>[10x]MSGTEEAILGGRDSHPAAGGGSVLCFGQCQYTAEEYQAIQKALRQRLGPEYISSRMAGGGQKVCYIEGHRVINLANEMFGYNGWAHSITQQNVDFVDLNNGKFYVGVCAFVRVQLKDGSYHEDVGYGVSEGLKSKALSLEKARKEAVTDGLKRALRSFGNALGNCILDKDYLRSLNKLPRQLPLEVDLTKAKRQDLEPSVEEARYNSCRPNMALGHPQLQQVTS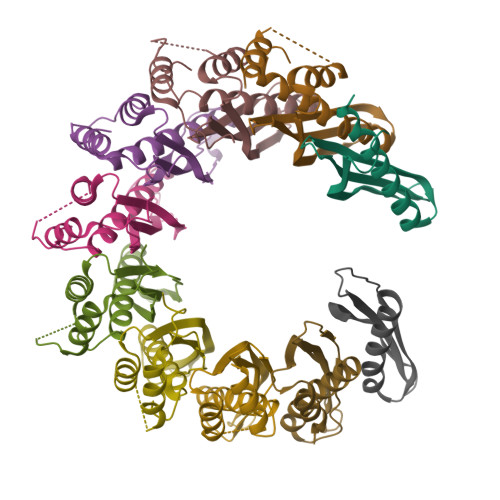PSRPSHAVIPADQDCSSRSLSSSAVESEATHQRKLRQKQLQQQFRERMEKQQVRVSTPSAEKSEAAPPAPPVTHSTPVTVSEPLLEKDFLAGVTQELIKTLEDNSEKWAVTPDAGDGVVKPSSRADPAQTSDTLALNNQMVTQNRTPHSVCHQKPQAKSGSWDLQTYSADQRTTGNWESHRKSQDMKKRKYDPS> KQLLSLKPISASDSLFISCTVFNSKGNIISMSEKFPKWSFLT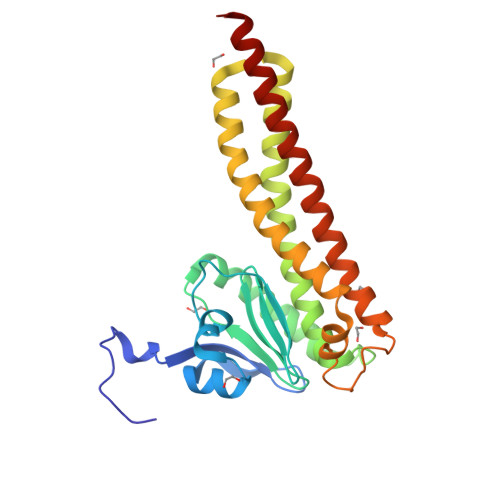EHSLFPRDLRKIDNSSIDIIPTIMCKPNCIVINLLHIKALIERDKVYVFDTTNPSAAAKLSVLMYDLESKLSSTKNNSQFYEHRALESIFINVMSALETDFKLHSQICIQILNDLENEVNRLKLRHLLIKSKDLTLFYQKTLLIRDLLDELLENDDDLANMYLTVKKSPKDNFSDLEMLIETYYTQCDEYVQQSESLIQDIKSTEEIVNIILDANRNSL>[4x]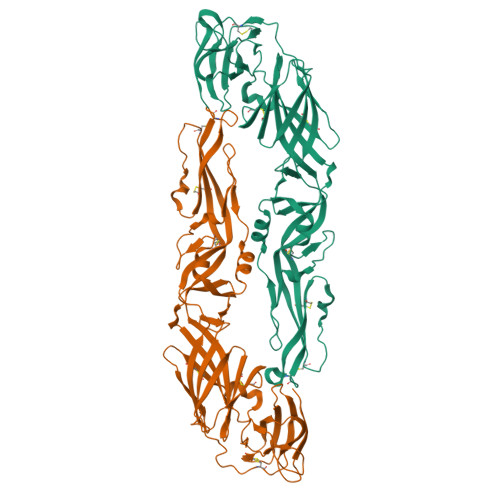AHCIGITDRDFIEGVHGGTWVSATLEQDKCVTVMAPDKPSLDISLQTVAIDGPAEARKVCYSAVLTHVKINDKCPSTGEAHLAEENDGDNACKRTYSDRGWGNGCGLFGKGSIVACAKFTCAKSMSLFEVDQTKIQYVIRAQLHVGAKQENWNTDIKTLKFDALSGSQEAEFTGYGKATLECQVQTAVDFGNSYIAEMEKDSWIVDRQWAQDLTLPWQSGSGGIWREMHHLVEFEPPHAATIRVLALGNQEGSLKTALTGAMRVTKDENDNNLYKLHGGHVSCRVKLSALTLKGTSYKMCTDKMSFVKNPTDTGHGTVVMQVKVPKGAPCKIPVIVADDLTAAVNKGILVTVNPIASTNDDEVLIEVNPPFGDSYIIVGTGDSRLTYQWHKEG> MADYKDDDDKSGPDEVDASGRGDTGLRKRREDEKSIQSQEPKTTSLQKELGLISGISIIVGTIIGSGIFVSPKSVLSNTEAVGPCLIIWAACGVLATLGALCFAELGTMITKSGGEYPYLMEAYGPIPAYLFSWASLIVIKPTSFAIICLSFSEYVCAPFYVGCKPPQIVVKCLAAAAILFISTVNSLSVRLGSYVQNIFTAAKLVIVAIIIISGLVLLAQGNTKNFDNSFEGAQLSVGAISLAFYNGLWAYDGWNQLNYITEELRNPYRNLPLAIIIGIPLVTACYILMNVSYFTVMTATELLQSQAVAVTFGDRVLYPASW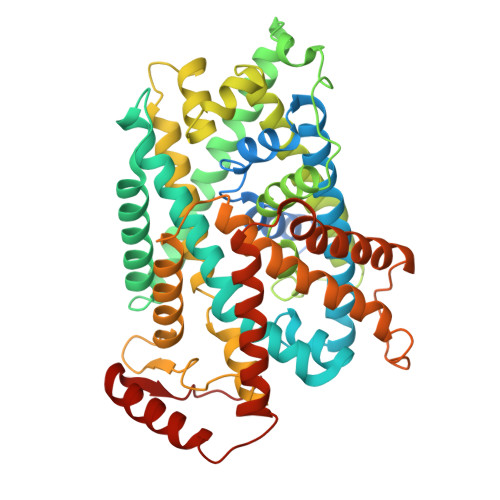IVPLFVAFSTIGAANGTCFTAGRLIYVAGREGHMLKVLSYISVRRLTPAPAIIFYGIIATIYIIPGDINSLVNYFSFAAWLFYGLTILGLIVMRFTRKELERPIKVPVVIPVLMTLISVFLVLAPIISKPTWEYLYCVLFILSGLLFYFLFVHYKFGWAQKISKPITMHLQMLMEVVPPEEDPE>[2x]GMPTRVIEDKGDMTPSFGIDDRIFLGEGLFETIRVNSSKPSFAYMHWERLGNSARQLGIPFEISFDDWFEHLIQKIQKDNLYHGGIKAILSGGPASRGLAERGQVSQLIFQTFNYSIQKHPVRLISINWLRDKANPLYQLKSVNYLEAIIAQRQAIAVGADDALFFNTENHVTETTCANLFLIENNILYTPRVEDGI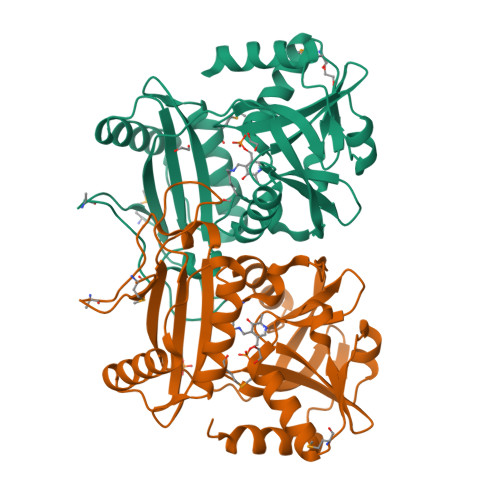LPGITRARLISHCQQHKMSVQEISLTKKRIEDADAVFLTNSLQGIRRVLSLDNIIFEVNHPIIDKLIFLLNQDES[(6-AMINO-9H-PURIN-9-YL)-[5-FLUORO-1,3-DIHYDRO-1-HYDROXY-2,1-BENZOXABOROLE]-4'YL]METHYL DIHYDROGEN PHOSPHATE | C17 H17 B F N5 O8 P | 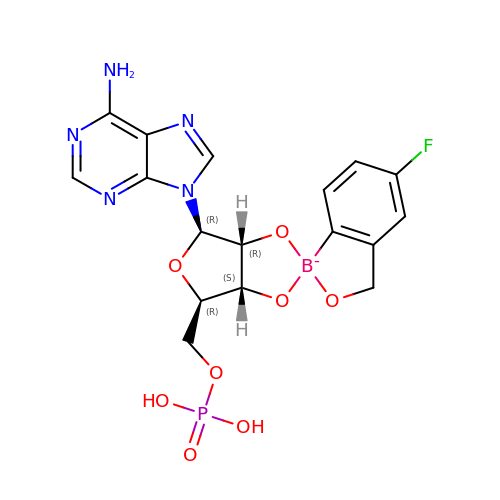ZLSXXTYLUMEAGG-LBTDBDNISA-N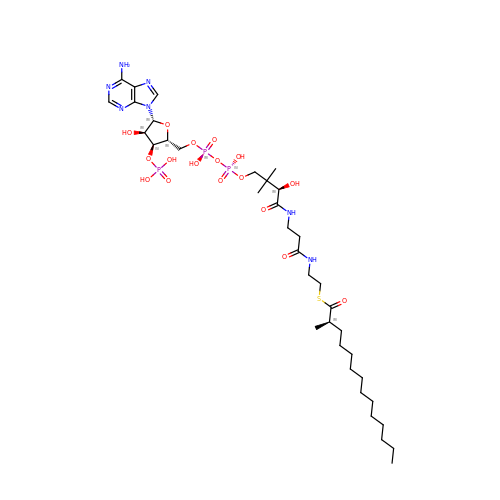(R)-2-METHYLMYRISTOYL-COENZYME A | C36 H64 N7 O17 P3 S | KJEFZXSIQKASDI-MOTPQXBDSA-N>SSQIRQNYSTDVEAAVNSLVNLYLQASYTYLSLGFYFDRDDVALEGVSHFFRELAEEKREGYERLLKMQNQRGGRALFQDIKKPAEDEWGKTPDAMKAAMALEKKLNQALLDLHALGSARTDPHLCDFLETHFLDEEVKLIKKMGDHLTNL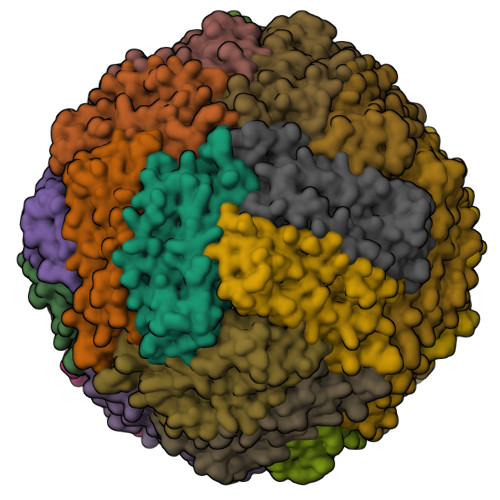HRLGGPEAGLGEYLFERLTLKHD[8x]>[2x]FFSCQRGYKGVWRGDGIMQTTCPCGAQITGHVKNGSMRIVGPRTCSNT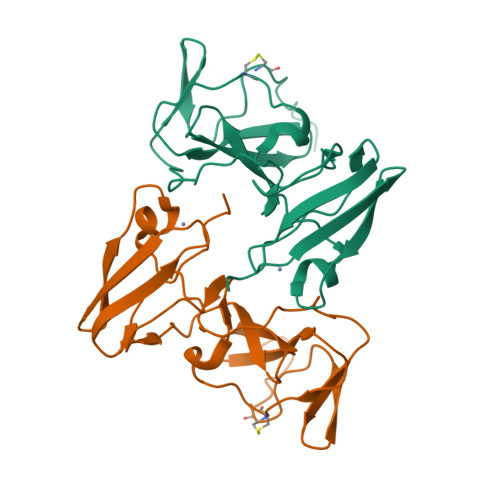WHGTFPINAYTTGPCTPSPAPNYSRALWRVAAEEYVEVTRVGDFHYVTGMTTDNVKCPCQVPAPEFFTEVDGVRLHRYAPACKPLLREEVTFLVGLNQYLVGSQLPCEPEPDVAV4-[7-[(dimethylamino)methyl]-2-(4-fluorophenyl)imidazo[1,2-a]pyridin-3-yl]pyrimidin-2-amine 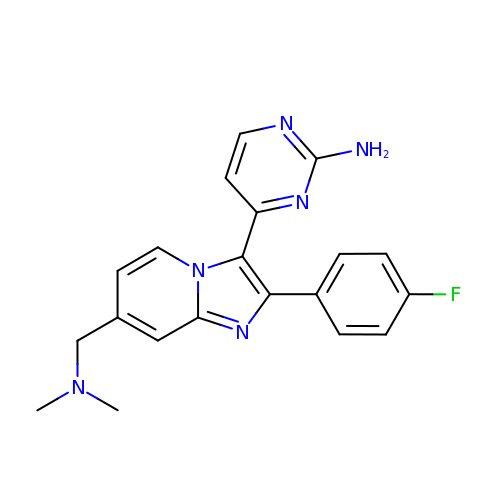| C20 H19 F N6 | HEPQZLAAWOEYMZ-UHFFFAOYSA-N> MSLRRGIYHIENAGVPSAIDLKDGSSSDGTPIVGWQFTPDTINWHQLWLAEPIPNVADTFTLCNLFSGTYMDLYNGSSEAGTAVNGWQGTAFTTNPHQLWTIKKSSDGTSYKIQ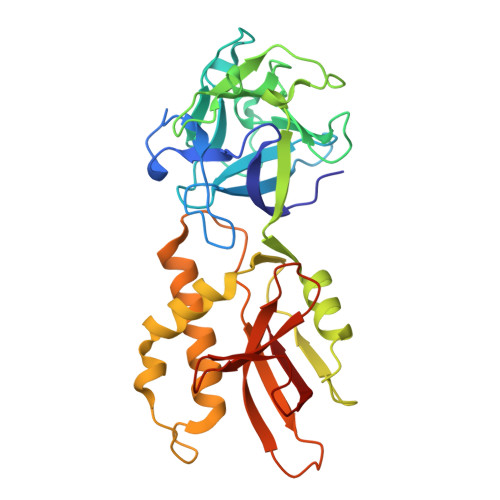NYGSKTFVDLVNGDSSDGAKIAGWTGTWDEGNPHQKWYFNRMSVSSAEAQAAIARNPHIHGTYRGYILDGEYLVLPNATFTQIWKDSGLPGSKWREQIYDADDFAIAMKAAVGKWGADSWKANGFAIFCGVMLGVNKAGDAAAAYNFTLTKDHADIVFFEPQNGGYLNDIGYDSYMAFY> MSDSPLSKRQKRKSAQEPELSLDQGDAEEDSQVENRVNLSENTPEPDLPALEASYSKSYTPRKLVLSSGENRYAFSQPTNSTTTSLHVPNLQPPKTSSRGRDHKSYSQSPPRSPGRSPTRRLELLQLSPVKNSRVELQKIYDRHQSSSKQQSRLFINELVLENFKSYAGKQVVGPFHTSFSAVVGPNGSGKSNVIDSMLFVFGFRANKMRQDRLSDLIHKSEAFPSLQSCSVAVHFQYVIDESSGTSRIDEEKPGLIITRKAFKNNSSKYYINEKESSYTEVTKLLKNEGIDLDHKRFLILQGEVENIAQMKPKAEKESDDGLLEYLEDIIGTANYKPLIEERMGQIENLNEVCLEKENRFEIVDREKNSLESGKETALEFLEKEKQLTLLRSKLFQFKLLQSNSKLASTLEKISSSNKDLEDEKMKFQESLKKVDEIKAQRKEIKDRISSCSSKEKTLVLERRELEGTRVSLEERTKNLVSKMEKAEKTLKSTKHSISEAENMLEELRGQQTEHETEIKDLTQLLEKERSILDDIKLSLKDKTKNISAEIIRHEKELEPWDLQLQEKESQIQLAESELSLLEETQAKLKKNVETLEEKILAKKTHKQELQDLILDLKKKLNSLKDERSQGEKNFTSAHLKLKEMQKVLNAHRQRAMEARSSLSKAQNKSKVLTALSRLQKSGRINGFHGRLGDLGVIDDSFDVAISTACPRLDDVVVDTVECAQHCIDYLRKNKLGYARFILLDRLRQFNLQPISTPENVPRLFDLVKPKNPKFSNAFYSVLRDTLVAQNLKQANNVAYGKKRFRVVTVDGKLIDISGTMSGGGNHVAKGLMKLGTNQSDKVDDYTPEEVDKIERELSERENNFRVASDTVHEMEEELKKLRDHEPDLESQISKAEMEADSLASELTLAEQQVKEAEMAYVKAVSDKAQLNVVMKNLERLRGEYNDLQSETKTKKEKIKGLQDEIMKIGGIKLQMQNSKVESVCQKLDILVAKLKKVKSASKKSGGDVVKFQKLLQNSERDVELSSDELKVIEEQLKHTKLALAENDTNMNETLNLKVELKEQSEQLKEQMEDMEESINEFKSIEIEMKNKLEKLNSLLTYIKSEITQQEKGLNELSIRDVT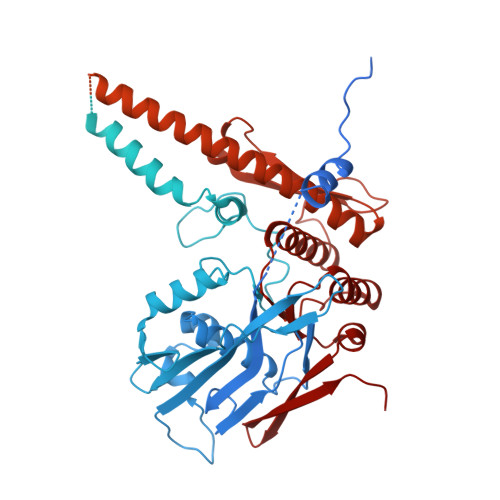HTLGMLDDNKMDSVKEDVKNNQELDQEYRSCETQDESEIKDAETSCDNYHPMNIDETSDEVSRGIPRLSEDELRELDVELIESKINELSYYVEETNVDIGVLEEYARRLAEFKRRKLDLNNAVQKRDEVKEQLGILKKKRFDEFMAGFNIISMTLKEMYQMITMGGNAELELVDSLDPFSEGVTFSVMPPKKSWRNITNLSGGEKTLSSLALVFALHKYKPTPLYVMDEIDAALDFRNVSIVANYIKERTKNAQFIVISLRNNMFELAQQLVGVYKRDNRTKSTTIKNIDILNRT>[2x]GPGMSASGSGDATLGIVHTLMCHRQGGESENFAKRAVESLVKKLKDKRDELDALITAVTSNGIQQSKCVTIARTLDGRLQVAGKKGFPHVIYSRIWRWPDLHKNELKHIKLCKFAFDLKLDHVCVNPYHYERVISPGYNVTDI

Smad proteins consist of an N-terminal MH1 domain, which binds to DNA, a linker region with phosphorylation sites for network regulatory inputs, and a C-terminal MH2 domain that is phosphorylated by the receptors and binds other Smad proteins, LDTFs, chromatin readers, and transcriptional co-activators and co-repressors. The receptors for TGF-β, nodal, activin, myostatin, and other family members are membrane serine/threonine kinases that phosphorylate and activate Smad2 and Smad3, whereas analogous receptors for the bone morphogenetic proteins (BMPs) preferentially phosphorylate and activate Smads 1, 5, and 8. These receptor-activated Smads (R-Smads) form heterotrimeric complexes with Smad4, which is required for the transcriptional regulation of most target genes. Focusing on the human and mouse Gsc promoter, here we identify specific Smad-binding GC-rich motifs and provide the X-ray crystal structures of Smad3 and Smad4 bound to several of these motifs. The structures determined here reveal that the β-hairpin is flexible and adaptable to bind with high-affinity several variants of the consensus sequence GGC(GC)|(CG), which we refer to as 5GC SBE.

We examined the recognition of the GGCGC site by the Smad4 MH1 domain of the Placozoa Trichoplax, metazoans whose bodies are composed by only four basic cell types and with one of the most divergent among the known Smad4 sequences relative to human Smad4. The crystal structure of the Trichoplax Smad4 MH1 domain bound to the GGCGC oligonucleotide reveals that this Smad4–DNA interaction is strictly conserved (diffraction data obtained at 2.43 Å, space group P212121, data collection, and statistics shown in Table 1). A superposition of the human Smad4 and Trichoplax Smad4 complexes shows that both complexes are very similar, and in particular the protein binding mode (Cα RMSD of 0.46 Å for 115 aligned residues). The few observed differences are concentrated in and around two loops that also contain most of the amino-acid sequence differences. Collectively, the results show that Smad4 proteins from highly divergent metazoan species interact with the GGCGC motif with similar binding affinity and similar structural contacts. The X-ray crystal structure of Trichoplax adhaerens Smad4 MH1 bound to one of these motifs indicates a high conservation of this interaction in metazoans.> LLRY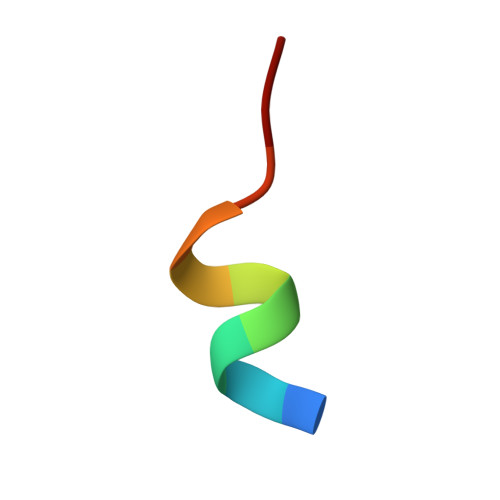LLDKDD2-hydroxyethyl hydrogen 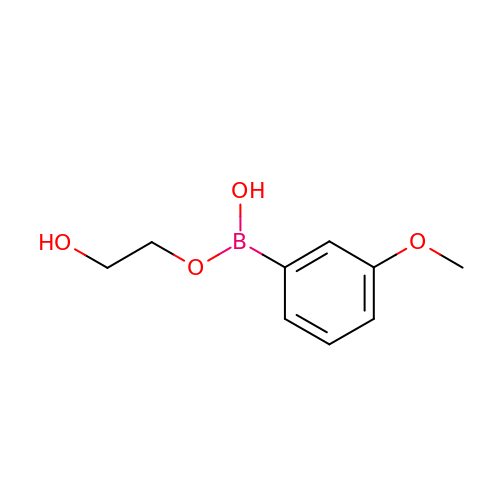(3-methoxyphenyl)boronate | C9 H13 B O4 | ZOVRPEMVSXQSPK-UHFFFAOYSA-N2-[4-(furan-2-ylcarbonyl)piperazin-1-yl]-6,7-dimethoxyquinazolin-4-amine 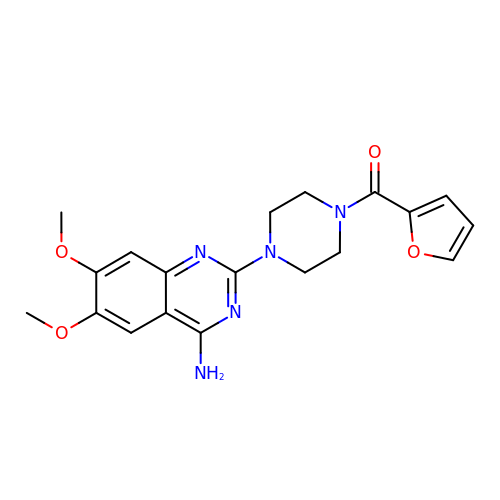| C19 H21 N5 O4 | IENZQIKPVFGBNW-UHFFFAOYSA-N> AGIDPNRIVALEWLPVELLLALGIVPYGVADTINYRLWVSEPPLPDSVIDVGLRTEPNLELLTEMKPSFMVWSAGYGPSPEMLARIAPGRGF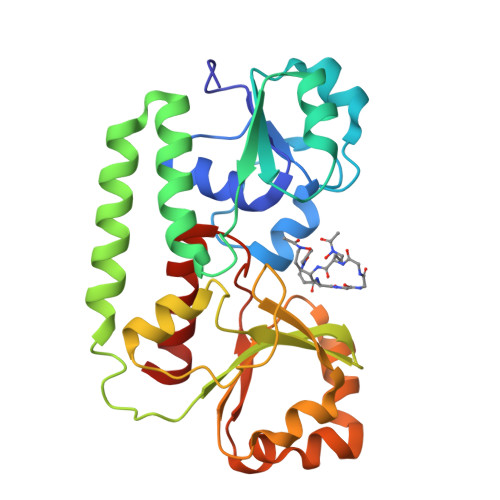NFSDGKQPLAMARKSLTEMADLLNLQSAAETHLAQYEDFIRSMKPRFVKRGARPLLLTTLIDPRHMLVFGPNSLFQEILDEYGIPNAWQGETNFWGSTAVSIDRLAAYKDVDVLCFDHDNSKDMDALMATPLWQAMPFVRAGRFQRVPAVWFYGATLSAMHFVRVLDNAIGGKA> MQNLKFAFSSIMAHKMRSLLTMIGIIIGVSSVVVIMALGDSL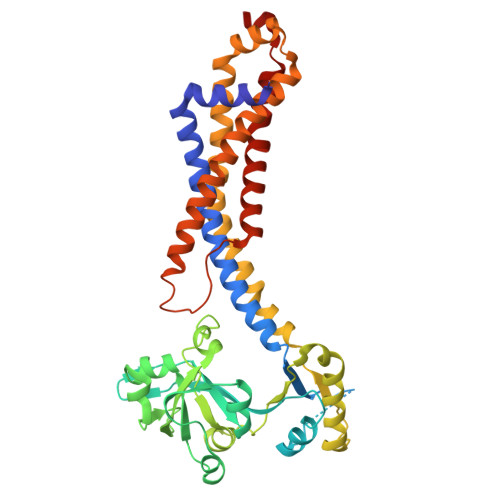SRQVNKDMTKSQKNISVFFSPKKSKDGSFTQKQSAFTVSGKEEEVPVEPPKPQESWVQEAAKLKGVDSYYVTNSTNAILTYQDKKVENANLTGGNRTYMDAVKNEIIAGRSLREQDFKEFASVILLDEELSISLFESPQEAINKVVEVNGFSYRVIGVYTSPEAKRSKIYGFGGLPITTNISLAANFNIDEIASIVFRVNDTSLTPTLGPELARKMTELAGLQQGEYQVADESVVFAEIQQSFSFMTTIISSIAGISLFVGGTGVMNIMLVSVTERTREIGLRKALGATRANILIQFLIESMILTLLGGLIGLTIASGLTALAGLLLQGLIEGIEVGVSIPVALFSLAVSASVGMIFGVLPANKASKLDPIEALRYE>SEISRQEFQRRRQALVEQMQPGSAALIFAAPEVTRSADSEYPYRQNSDFWYFTGFNEPEAVLVLIKSDDTHNHSVLFNRVRDLTAEIWFGRRLGQDAAPEKLGVDRALAFSEINQQLYQLLNGLDVVYHAQGEYAYADVIVNSALEKLRKGSRQNLTAPATMIDWRPVVHEMRLFKSPEEIAVLRRAGEITAMAHTRAMEKCRPGMFEYHLEGEIHHEFNRHGARYPSYNTIVGSGENGCILHYTENECEMRDGDLVLIDAGCEYKGYAGDITRTFPVNGKFTQAQREIY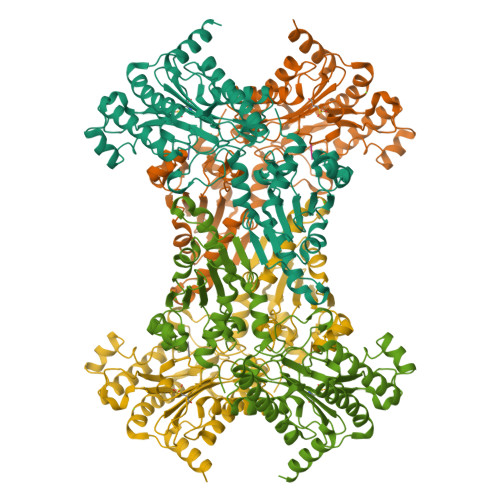DIVLESLETSLRLYRPGTSILEVTGEVVRIMVSGLVKLGILKGDVDELIAQNAHRPFFMHGLSHWLGLDVHDVGVYGQDRSRILEPGMVLTVEPGLYIAPDAEVPEQYRGIGIRIEDDIVITETGNENLTASVVKKPEEIEALMVAARKQ[4x];>[4x]VPL> HTVE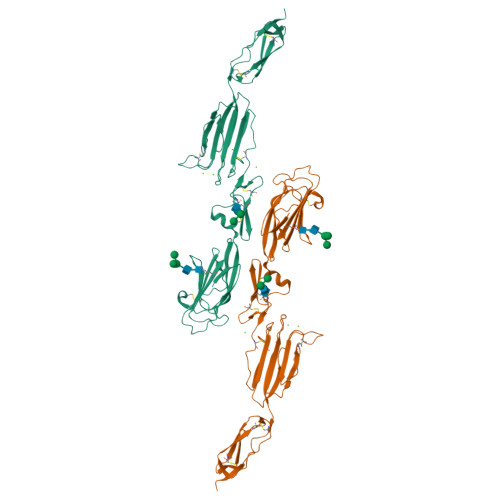LNNMFGQIQSPGYPDSYPSDSEVTWNITVPDGFRIKLYFMHFNLESSYLCEYDYVKVETEDQVLATFCGRETTDTEQTPGQEVVLSPGSFMSITFRSDFSNEERFTGFDAHYMAVDVDECKEREDEELSCDHYCHNYIGGYYCSCRFGYILHTDNRTCRVECSDNLFTQRTGVITSPDFPNPYPKSSECLYTIELEEGFMVNLQFEDIFDIEDHPEVPCPYDYIKIKVGPKVLGPFCGEKAPEPISTQSHSVLILFHSDNSGENRGWRLSYRAAGNECPELQPPVHGKIEPSQAKYFFKDQVLVSCDTGYKVLKDNVEMDTFQIECLKDGTWSNKIPTCKKNEIDLESELKSEQVTE> CCGAGTCCTA;> CTCAACTCGG;> TCGGCCTGAG;> TAGGGGC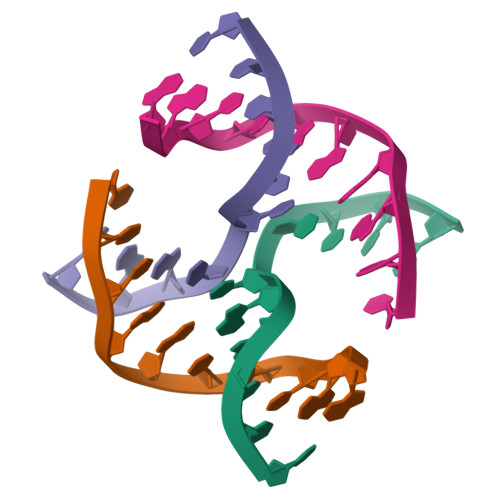CGA> MSDVAIVKEGWLHKRGEYIKTWRPRYFLLKNDGTFIGYKERPQDVDQREAPLNNFSVAQCQLMKTERPRPNTFIIRCLQWTTVIEATFHVETPEEREEWTTAIQTVADGLKKQEEEEMDFR

The Ser/Thr protein kinase Akt1 (termed Akt in the present work) and its paralogs Akt2 and Akt3 serve as key effectors in the PI3-kinase/Akt signaling pathway to regulate cell survival, proliferation, and metabolism by phosphorylating a variety of protein substrates. Akt is a 480 amino acid protein comprised of an N-terminal pleckstrin homology (PH) domain, a central kinase domain, and a regulatory C-tail. Regulation of Akt’s activity involves an autoinhibitory intramolecular interaction between its pleckstrin homology (PH) domain and its kinase domain that can be relieved by C-tail phosphorylation. Akt’s PH domain shows high affinity and selectivity for the phospholipid, phosphatidylinositol 3,4,5-triphosphate (PIP3) using its positively charged basic residues including Lys14, Arg23, Arg25, and perhaps to a limited extent Arg86.

Here, we discover unexpectedly that a single mutation R86A Akt exhibits intensified autoinhibitory features with enhanced PH domain-kinase domain affinity. Despite the NMR HSQC analysis suggesting the possibility of structural perturbations induced by R86A mutation, the X-ray structure of the R86A PH domain revealed very high concordance between the WT and R86A PH domain structures, with an overall RMSD of 0.198 for main chain atoms. The structure of the R86A mutant was determined in the same crystal lattice as the WT protein, and their main chain conformations are essentially identical. In fact, apart from the mutated Arg86 residue, only the side chains of Glu17 and Tyr18 showed significant structural changes in the R86A X-ray structure. By contrast, in the R86A PH domain, the Glu17 side chain rotates away from Ala86 and the side chain of Lys14, and this rearrangement appears to induce an alternate side chain rotamer for Tyr18. Paradoxically, breaking the Arg86-Glu17 hydrogen bond by R86A mutation sharply increases PH domain stability and promotes a Tyr18 rotamer which enhances the binding of the PH domain to the kinase domain. The R86A PH domain displayed an approximately threefold greater binding affinity (KD 37 μM) toward the kinase domain than the WT PH domain (KD 107 μM), supporting the idea that R86A mutation stabilizes the autoinhibited Akt state by promoting the PH-kinase interdomain interaction. Differential scanning fluorimetry revealed that R86A has increased melting temperature (51±1°C) compared to WT PH domain (42±1°C). Notably, these R86A-driven CSPs have a higher magnitude compared to the CSPs due to the interaction with the kinase domain. This supports our hypothesis that the R86A PH domain is preorganized in a rigid, stable, conformation suited for tight inhibitory interaction with the kinase domain.>[4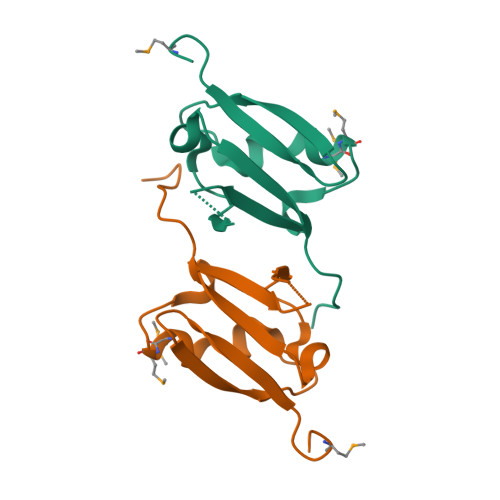x]MGHHHHHHSHMQKPIVRVFLPNKQRTVVPARCGVTVRDSLKKALMMRGLIPECCAVYRIQDGEKKPIGWDTDISWLTGEELHVEVLENVPLTTHNF>MGNRGMEDLIPLVNRLQDAFSAIGQNADLDLPQIAVVGGQSAGKSSVLENFVGRDFLPRGSGIVTRRPLVLQLVNATTEYAEFLHCKGKKFTDFEEVRLEIEAETDRVTGTNKGISPVPINLRVYSPHVLNLTLVDLPGMTKVPVGDQPPDIEFQIRDMLMQFVTKENCLILAVSPANSDLANSDALKVAKEVDPQGQRTIGVITKLDLMDEGTDARDVLENKLLPLRRGYIGVVNRSQKDIDGKKDITAALAAERKFFLSHPSYR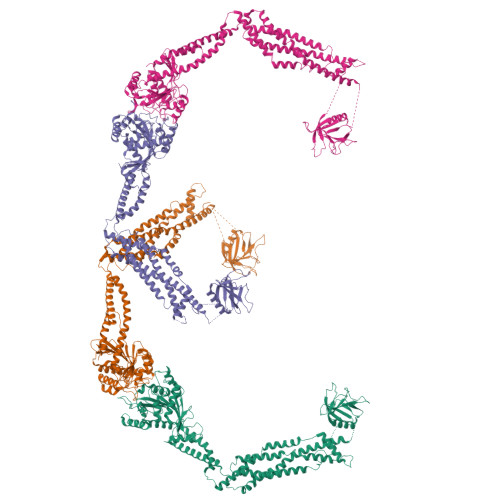HLADRMGTPYLQKVLNQQLTNHIRDTLPGLRNKLQSQLLSIEKEVEEYKNFRPDDPARKTKALLQMVQQFAVDFEKRIEGSGDQIDTYELSGGARINRIFHERFPFELVKMEFDEKELRREISYAIKNIHGIRTGLFTPDMAFETIVKKQVKKIREPCLKCVDMVISELISTVRQCTKKLQQYPRLREEMERIVTTHIREREGRTKEQVMLLIDIELAYMNTNHEDFIGFANAQQRSNQMNKKKTSGNQDEILVIRKGWLTINNIGIMKGGSKEYWFVLTAENLSWYKDDEEKEKKYMLSVDNLKLRDVEKGFMSSKHIFALFNTEQRNVYKDYRQLELACETQEEVDSWKASFLRAGVYPERVGDKEKASETEENGSDSFMHSMDPQLERQVETIRNLVDSYMAIVNKTVRDLMPKTIMHLMINNTKEFIFSELLANLYSCGDQNTLMEESAEQAQRRDEMLRMYHALKEALSIIGDINTT[4x]>GPMNNDEQLEFLINYLLDERSESIDIPKTFSEKRNLLRSLMNMRHPSNISEEFLRIQDEFLSRETANKNLTSVEDISLSSGKIMLWQGDITTLSADAIVNAANSKLLGCFIPMHNCIDNIIHSASGLQLREECNRMIMLQGGDEDVGKAKITNAYNLPSKYVVHTVGPSIERGMRVSSDDVKKLERCYNSCLELASEYKLNSIAFCCISTGVFNFPQKKAAEIAIRTVKDFLNSNETSLNHIIFDVFTDKDYDIYKKLLFGN[2x]

In some pathogenic microbes, the response to oxidative stress is controlled by a SirTM/zinc-containing macrodomain (Zn-Macro) pair responsible for establishment and removal of the modification, respectively. Strikingly, however, the “catalytic loop” found in all other MacroD-type enzymes (also termed “loop 1”) is replaced with and extended loop containing the zinc-coordinating Cx(4)HxC motif, here termed the Zn-loop. To gain a closer understanding of the functional role of the 3α-bundle and coordinated Zn2+ ion, we solved structures from the three sub-branches of Zn-Macros namely from S. aureus (SauMacro), Methanobrevibacter oralis (MorMacro), and macrodomain-fused SirTM protein (Mfs1) from Fusarium oxysporum f.sp. cubense race 1 (Foc1Mfs1) in their apo form as well as of S. pyogenes (SpyMacro) and MorMacro bound to ADP-ribose (ADPr). In all structures, the Zn2+ ion is tetrahedrally coordinated with three metal-coordination residues within the Zn-loop, while the fourth coordination-contact is exchangeable and is provided by either ADPr, a water molecule, or a symmetry-related protomer within the crystal.

However, our data do not support this binding mode: first, the different orientation of the diphosphate-binding loop in our apo structures shortens the cavity, which would sterically hinder the binding of the dithiolane moiety. Surprisingly, neither MorMacro, which arises from a minimal operon containing only the Zn-Macro/SirTM pair, nor Zn-Macros derived from Msf1 fusion proteins could demodify SpyGcvH-L. In contrast, all Zn-Macros could demodify Glu-/Asp-ADP-ribosylated PARP1 E988Q. On the other hand, the absence of positive interaction surfaces in the other family members of the Zn-Macro family (having neutral to negative surfaces) might provide an energetic barrier to GcvH-L binding and explain the absence of activity from these macrodomains.>MGSSHHHHHHSSGLVPAGSHMQLVSNGFEVNLPDQVEVIVRDLPDPSKVKEERTRLMGYWFVHWFDGKLFHLRIKAGGPNVDGEHRAIRTAEHPWLLRARLDDALEEALPKYAAVKKRPFTFLAQKDELIDAAATAAGLSHRLLNSFKVIPRFALSPKIYEPVDGTTRVGVFVTIGMRYDIEASLRDLLEAGIDLRGMYVVRRKRQPGERGLLGRVRAISDDMVQLFEETDLASVNVNDAKLEGSKENFTRCLSALLGHNYKKLLNALDDQEAGYRTGPRFDDAVRRMGEFLAKKPIRLADNINAQVGDRIVFSNEGQARNVRLAPKVEYVFDRTGAKSAEYAWRGLSQFGPFDRPSFANRSPRILVVYPSSTQGKVENFLSAFRDGMGSNYSGFSKGFVDLMGLTKVEFVMCPVEVSSADRNGAHTKYNSAIEDKLAGAGEVHAGIVVLFEDHARLPDDRNPYIHTKSLLLTLGVPTQQVRMPTVLLEPKSLQYTLQNFSIATYAKLNGTPWTVNHDKAINDELVVGMGLAELSGSRTEKRQRFVGITTVFAGDGSYLLGNVSKECEYEGYSDAIRESMTGILRELKKRNNWRPGDTVRVVFHAHRPLKRVDVASIVFECTREIGSDQNIQMAFVTVSHDHPFVLIDRSERGLEAYKGSTARKGVFAPPRGAISRVGRLTRLLAVNSPQLIKRANTPLPTPLLVSLHPDSTFKDVDYLAEQALKFTSLSWRSTLP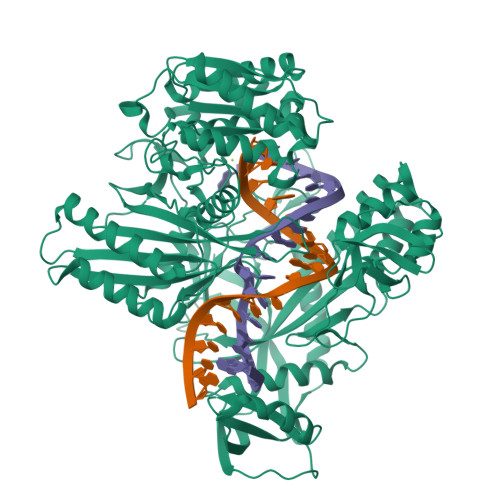AATPVTIFYSERIAELLGRLKSIPNWSSANLNIKLKWSRWFL[2x]Cystathionine beta-synthase (CBS) is an essential metabolic enzyme across all domains of life for the production of glutathione, cysteine, and hydrogen sulfide. Human CBS adopts a unique multi-domain structure: an N-terminal haem binding domain (residues 38–74), a central PLP-dependent catalytic domain (CD, residues 75–382), and a C-terminal regulatory domain (RD, residues 411–551)5,11,12. The RD adopts the evolutionarily conserved Bateman module, consisting of two tandem CBS motifs (CBS-1 and CBS-2) and a surface-exposed loop (residues 516–525) extending from a CBS-2 motif. Here we show using cryo-electron microscopy that full-length human CBS in the basal and SAM-bound activated states polymerises as filaments mediated by a conserved regulatory domain loop.

To this end, cryo-EM was used to analyse CBSFL-CHis in the presence of SAM. Micrographs showed that CBS retains a filamentous architecture in the presence of SAM but with a significantly altered morphology, as shown by 2D classes. Through helical refinement, we generated a global map at 4.0 Å resolution which reveals a central helical stalk decorated with highly flexible lobes. The overall morphology of the resulting filament is drastically different in comparison to the basal state, as reflected by the 66% increase in twist (−178.6°) and 10% decrease in rise (46.9 Å) of the filament in the presence of SAM. In the context of the full-length enzyme elucidated here, the SAM-mediated conformational change creates a central filament stalk composed of repeating units of the SAM-bound RD dimer, arranged in an antiparallel “daisy-chain” like fashion due to the interactions of the loop 516–525 with the neighbouring subunit. The central filament stalk is decorated by highly flexible CDs, where the active site entrance loops are free to open and hence increase the accessibility for substrates. Comparing our basal and activated filaments, the SAM-mediated conformational change to the RD is highly agreeable with that observed in the crystal structures of CBSΔ516–525 dimers where there is a relative 18° rotation between the CBS-1 and CBS-2 motifs caused by SAM binding. In our activated filament maps, ligand density was present for SAM only at the S2 site. No apparent and interpretable density was found for SAM at the S1 site nor at the filament interfaces. Overall, our data suggests that CBS likely binds SAM in a 1:1 manner and that our observed filament structures only reveal S2 as a SAM binding site.

>MPSETPQAEVGPTGCPHRSGPHSAKGSLEKGSPEDKEAKEPLWIRPDAPSRCTWQLGRPASESPHHHTAPAKSPKILPDILKKIGDTPMVRINKIGKKFGLKCELLAKCEFFNAGGSVKDRISLRMIEDAERDGTLKPGDTIIEPTSGNTGIGLALAAAVRGYRCIIVMPEKMSSEKVDVLRALGAEIVRTPTNARFDSPESHVGVAWRLKNEIPNSHILDQYRNASNPLAHYDTTADEILQQCDGKLDMLVASVGTGGTITGIARKLKEKCPGCRIIGVDPEGSILAEPEELNQTEQTTYEVEGIGYDFIPTVLDRTVVDKWFKSNDEEAFTFARMLIAQEGLLCGGSAGSTVAVAVKAAQELQEGQRCVVILPDSVRNYMTKFLSDRWMLQKGFLKEEDLTEKKPWWWHLRVQELGLSAPLTVLPTITCGHTIEILREKGFDQAPVVDEAGVILGMVTLGNMLSSLLAGKVQPSDQVGKVIYKQFKQIRLTDTLGRLSHILEMDHFALVVHEQIQYHSTGKSSQRQMVFGVVTAIDLLNFVAAQERDQKAAHHHHHH[10x]ethyl 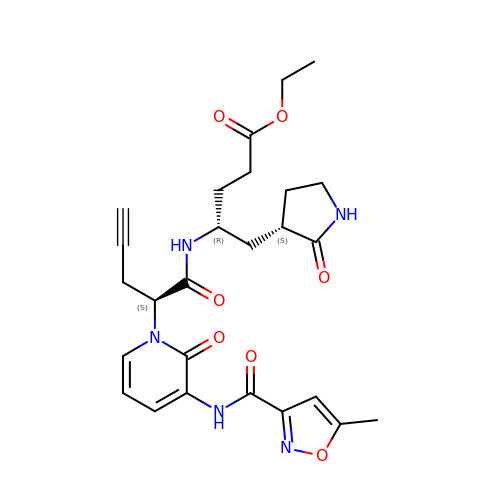(4R)-4-({(2S)-2-[3-{[(5-methyl-1,2-oxazol-3-yl)carbonyl]amino}-2-oxopyridin-1(2H)-yl]pent-4-ynoyl}amino)-5-[(3S)-2-oxopyrrolidin-3-yl]pentanoate | C26 H31 N5 O7 | WVFVHUYBPRBKRA-UEXGIBASSA-N>GGCAGCAG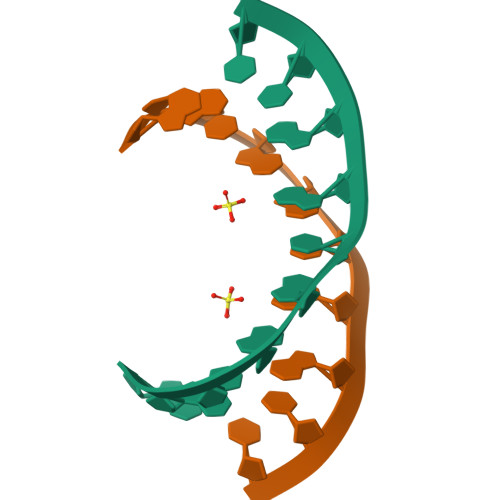CC[6x]> GAMGGPKPGGGPGLSTPGGHPKPPHRGGGEPRGGRQHHPPYHQQHHQGPPPGGPGGRSEEKISDSEGFKANLSLLRRPGEKTYTQRCR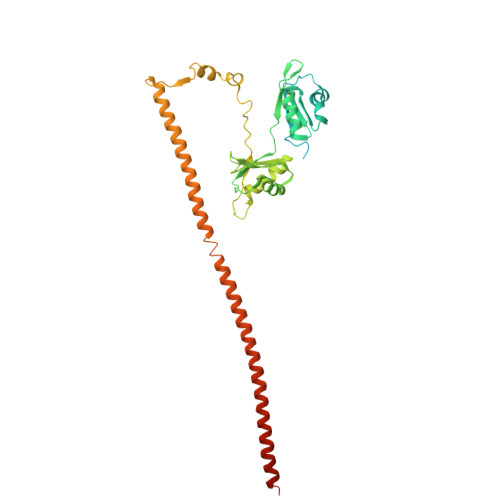LFVGNLPADITEDEFKRLFAKYGEPGEVFINKGKGFGFIKLESRALAEIAKAELDDTPMRGRQLRVRFATHAAALSVRNLSPYVSNELLEEAFSQFGPIERAVVIVDDRGRSTGKGIVEFASKPAARKAFERCSEGVFLLTTTPRPVIVEPLEQLDDEDGLPEKLAQKNPMYQKERETPPRFAQHGTFEYEYSQRWKSLDEMEKQQREQVEKNMKDAKDKLESEMEDAYHEHQANLLRQDLMRRQEELRRMEELHNQEMQKRKEMQLRQEEERRRREEEMMIRQREMEEQMRRQREESYS(1R,2S,3R,4S,5R,6R)-5-(8-azidooctylamino)-6-(hydroxymethyl)cyclohexane-1,2,3,4-tetrol | C15 H30 N4 O4 | 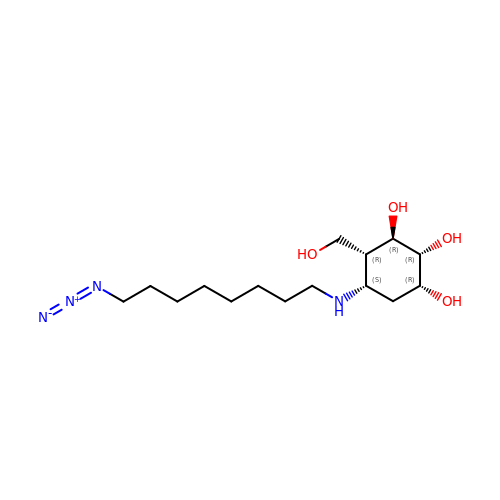GOBIPKNKUJPACR-VQJWOFKYSA-N> MKLAVAALLVASAAAFAPAPASKASTSLKVSEIELGVTEPLGVYDPLGWLESEPEAFERRRAVERKHGRVAMAAVVGTIVHNNHIVFDGYLSPSNNLKFSDIPTGVDGIRAIPTAGLAQILAFFALVELAWMPASKYDGDYG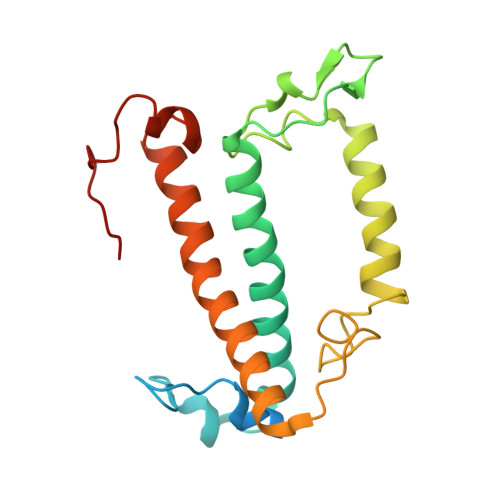VGYFGTDIKDPEEKARKLNVELNNGRAAMMGIMGNMVAEVLTGQTMYEQYASGHISPFGDGQGVF[1-(1-METHYL-4,5-DIOXO-PENT-2-ENYLCARBAMOYL)-2-PHENYL-ETHYL]-CARBAMIC ACID BENZYL ESTER | C23 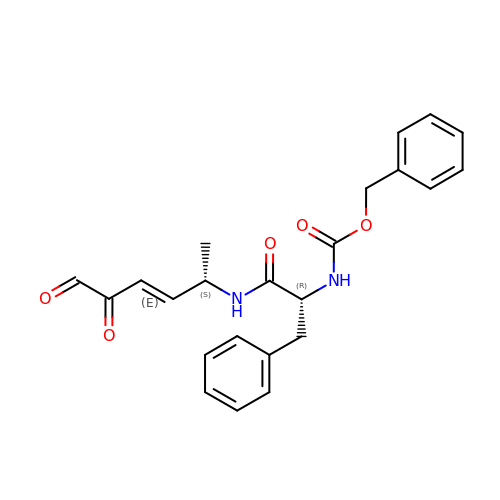H24 N2 O5 | NOXVWFAAXREWMI-GURWAVDKSA-N>[4x]GHMSPNYDKWEMERTDITMKHKLGGGQYGEVYEGVWKKYSLTVAVKTLKEDTMEVEEFLKEAAVMKEIKHPNLVQLLGVCTREPPFYIITEFMTYGNLLDYLRECNRQEVNAVVLLYMATQISSAMEYLEKKNFIHRDLAARNCLVGENHLVKVADFGLSRLMTGDTYTAHAGAKFPIKWTAPESLAYNKFSIKSDVWAFGVLLWEIATYGMSPYPGIDLSQVYELL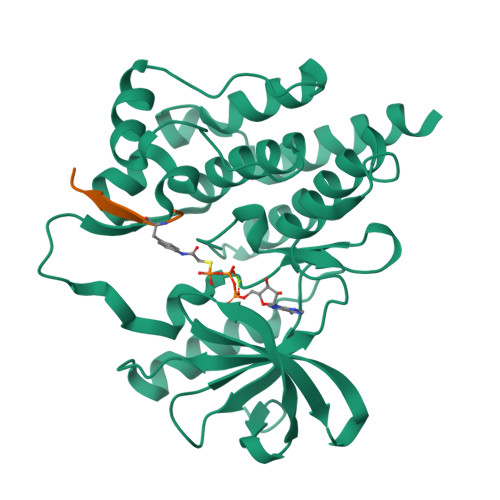EKDYRMERPEGCPEKVYELMRACWQWNPSDRPSFAEIHQAFETMFQESSISDEVEKELGK;>[4x]AEEEIFGEFEAKK>MQDITMQWYQQLQDASMQCVLTFEGLTNSKDSQAKKIKMDLQKAATIPVSQISTIAGSKLKEIFDKIHSLLSGKPVQSGGRSVSVTLNPQGLDFVQYKLAEKFVKQGEEEVASHHEAAFPIAVVASGIWELHPRVGDLILAHLHKKCPYSVPFYPTFKEGMALEDYQRMLGYQVKDSKVEQQDNF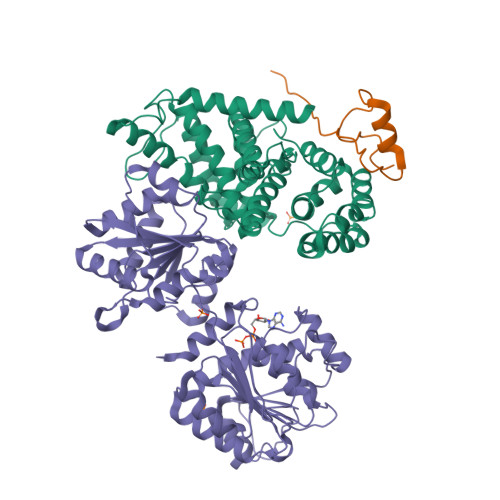LKRMSGMIRLYAAIIQLRWPYGNRQEIHPHGLNHGWRWLAQILNMEPLSDVTATLLFDFLEVCGNALMKQYQVQFWKMLILIKEDYFPRIEAITSSGQMGSFIRLKQFLEKCLQHKDIPVPKGFLTSSFWRS[2x];>[2x]GPSGSIIATDNVLFTPRDKLTVEELEQFQSKKFTLGKIPLKPPPLELLNV;>GPHMEDRAAQSLLNKLIRSNLVDNTNQVEVLQRDPNSPLYSVKSFEELRLKPQLLQGVYAMGFNRPSKIQENALPLMLAEPPQNLIAQSQSGTGKTAAFVLAMLSQVEPANKYPQCLCLSPTYELALQTGKVIEQMGKFYPELKLAYAVRGNKLERGQKISEQIVIGTPGTVLDWCSKLKFIDPKKIKVFVLDEADVMIATQGHQDQSIRIQRMLPRNCQMLLFSATFEDSVWKFAQKVVPDPNVIKLKREEETLDTIKQYYVLCSSRDEKFQALCNLYGAITIAQAMIFCHTRKTASWLAAELSKEGHQVALLSGEMMVEQRAAVIERFREGKEKVLVTTNVCARGIDVEQVSVVINFDLPVDKDGNPDNETYLHRIGRTGRFGKRGLAVNMVDSKHSMNILNRIQEHFNKKIERLDTDDLDEIEKIAN[2x]> MTQELGNANFENFIGATEGFSEIAYQFTSHILTLGYAVMLAGLLYFILTIKNVDKKFQMSNILSAVVMVSAFLLLYAQAQNWTSSFTFNEEVGRYFLDPSGDLFNNGYRYLNWLIDVPMLLFQILFVVSLTTSKFSSVRNQFWFSGAMMIITGYIGQFYEVSNLTAFLVWGAISSAFFFHILWVMKKVINEGKEGISPAGQKILSNIWILFLIS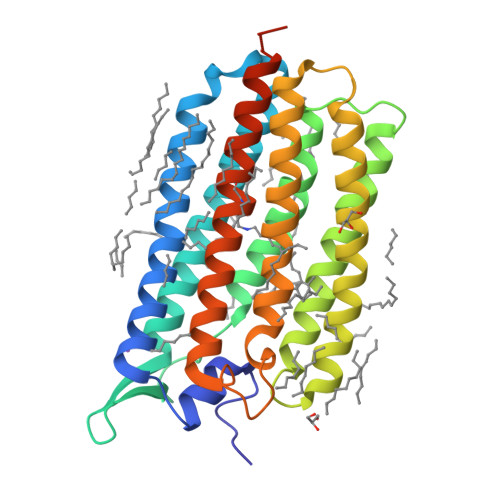WTLYPGAYLMPYLTGVDGFLYSEDGVMARQLVYTIADVSAKVIYGVLLGNLAITLSKNKELVEANSLEHHHHHH>GDGAGASRQRKLEALIRDPRSPINVESLLDGLNSLVLDLDFPALRKNKNIDNFLNRYEKIVKKIRGLQMKAEDYDVVKVIGRGAFGEVQLVRHKASQKVYAMKLLSKFEMIKRSDSAFFWEERDIMAFANSPWVVQLFYAFQDDRYLYMVMEYMPGGD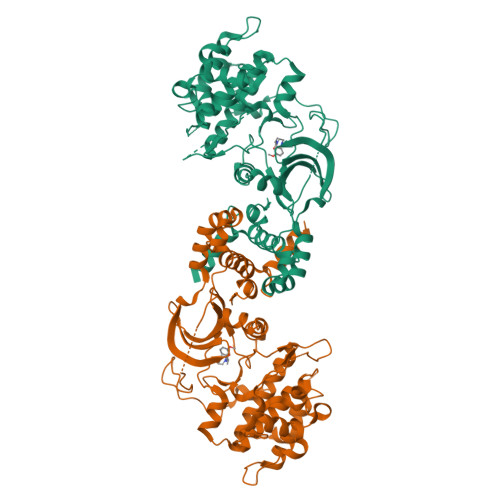LVNLMSNYDVPEKWAKFYTAEVVLALDAIHSMGLIHRDVKPDNMLLDKHGHLKLADFGTCMKMDETGMVHCDTAVGTPDYISPEVLKSQGGDGFYGRECDWWSVGVFLYEMLVGDTPFYADSLVGTYSKIMDHKNSLCFPEDAEISKHAKNLICAFLTDREVRLGRNGVEEIRQHPFFKNDQWHWDNIRETAAPVVPELSSDIDSSNFDDIEDDKGDVETFPIPKAFVGNQLPFIGFTYYR[4x]>NGLTYCTHASGFSFNPQTADAGTSMNVVTEQIYNKLFDIKNHSATLTPMLAQSYSISADGKEILLNLRHGVKFHQTPWFTPTRDFNAEDVVFSINRVLGHNTYLPTLAEANVTYSNPQYKVFHEQARKVRFPYFDSIKLNEKIKSVTALSPYQVKIELFAPDSSILSHLASQYAIIFSQEYAYQLSADDNLAQLDTHPVGTGPYQVKDYVYNQYVRLVRNENYWKKEAKIEHIIVDLSTDRSGRLVKFFNNECQIASYPEVSQIGLLKNDDKHYYMQSTDGMNLAYLAFNFDKPLMRDHEIRAAISQSLNRARIIHSIYHNTATVANNIIPEVSWASTVNTPEFEFDYHPKIAKNKLADKNLLLNLWVINEEQVYNPAPFKMAEMIKWDLAQAGVKVKVRAVTRPFLTAQLRNQSENYDLILSGWLAGNLDPDGFMRPILSCGTKNELTNLSNWCNEEFDQFMDRAITTSHLSSRAKAYNEAQELVLRELPIIPIANVKRILVANSRVKGVKMTPFGSLDFSTLYFI[2x]

Important for NTHi survival, colonization and persistence in vivo is the Sap (sensitivity to antimicrobial peptides) ABC transporter system. An essential system for NTHi survival and persistence in vivo is the Sap (sensitivity to antimicrobial peptides) transporter. This multi-component system uses a periplasmic protein (SapA) to bind and deliver substrates to the heterodimeric inner membrane-associated Sap permease (SapBC). The Sap ABC transporter is completed by two membrane-associated nucleotide-binding proteins (SapD & SapF) that hydrolyze ATP to provide energy for substrate transport across the bacterial inner membrane. The structure confirmed the classification of SapA into the Substrate Binding Protein (SBP) superfamily, as was predicted from sequence analysis.

SapA was successfully crystallized in an open (no ligand) and closed conformation with an endogenous ligand in the binding cavity. As a comparison, the distance between Asp 222 and Val 435, residues that respectively reside near to the termini of lobes I and II, are 35 Å apart in SapAclosed and over 40 Å apart in SapAopen. A transition from the open to closed state requires a 15.6° rotation around the axis bisecting domains I and II. Conformational shifts such as these are characteristic of the SBP superfamily upon binding/release of their cognate ligand and have been described as a “Venus flytrap” mechanism. In SapAclosed, the lobes enclose a cavity with two narrow openings to the protein surface. Difference electron density (Fo—Fc) became apparent within this cavity during the later stages of refinement. This additional density was not observed in SapAopen. Identical RNA binding was observed at the same site in both SapAclosed and SapAopen and therefore did not appear to affect the overall conformation of the protein. The antisense strand is provided by a SapA symmetry mate. Furthermore, although definitive electron density is only present for a 19 bp stretch RNA, inspection of the symmetry neighbors indicates that the RNA strands extend across asymmetric units, forming a matrix within the crystal.> MAQRVKITTTATPGEIELAFEDTGTGLPVLLVHGFPLDRTMWKAQREELCDEFRVIVPDLRGFGESQVIPGVATMEAMADDLAGLCNHLG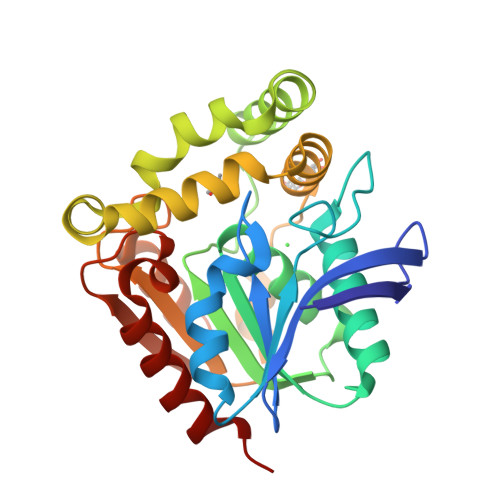LTGKIVLGGLSMGGYVAFAFARKYRDRLAGLILCDTRARPDSPEAKENRRRVAERVRREGPGFIAEEMIPRLCCESTFRNHPEVIEKIRQMILSAPPEGVAAAALGMAERPDSTDLLPALSCPTLVLVGQFDAISPPEEMEAMARTIPQSQFVVIPDAGHLPPMEQPERVTQAIREWLRKVHTE> MVVKASGGSSVARPQLYQTVPVSTIIQAEQQDRFLNRGELDELAVYLRSGAKRLEIATTLTRNADIIVSRAANRIFVGGSPMAFLSRPQTEEAPQFTTGARGEAIDIKEAMKLGTATYVDTRGGFLEGLRSIFSASSGGAPVGFKPINIARYGPARMEKSLRDLDWFLRYTTYAIVAGDPNILAVNTRGLREIIEAACSSDATIAALQEMRRAALSYFEKDAEAKGIVETYFDVLINEFIAPAPSDKVRQRNSTDLQGLQLPQIYFNAAERRPKFVMKPGLSA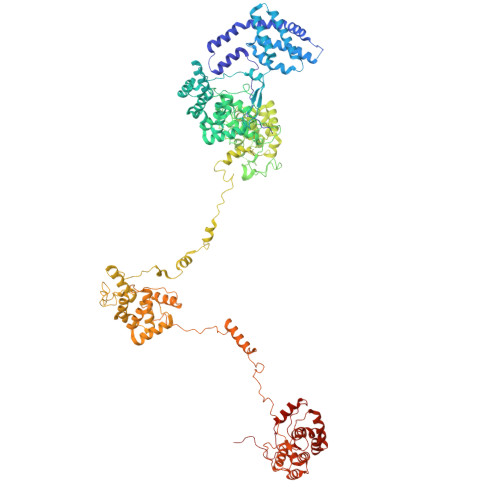AEKNEVVKAAYRQIFERDISRAYGLGISDLESKVKNGSISMKEFIRQLAKSPLYRKNFYEPYINSRALELAFRHILGRGPSSREEVQTYFAIISKGGLPALVDALVDSKEYSDYFGEETVPYLRGLGQEAQECRNWGAQQDLFKYSAPFRKVPQFITTFAAQDQPLPDQHPYGSGNDPLEIQFGAIFPKEKKNPSARPQPFNKDTRRILIARGPGINNQVSNPGARGLTPGTLGPKVFKLDQLPSINARIGKRSIATGTDSVKFAESSTQRVIRAAYLQVFGRDVYEGQRQKVAEIKLENGEISVREFVRILAKSNLFRSLYWTPLYVTKAIEYIHRRLLGRPTYGRQEMNAYFDIASKKGLYGLVDAIIDSQEYSEAFGEDTVPYERYITPQGLALRSLRVGTIGETGVPPEKEETPRFVELGAVTELRTEPAIQFRANQGVSKRREQTKVFKLTDLNDKQNLQLVIQAAYRQVFERDVAPYIVRDEFTALESKLSNGEITLKEFIEALGCSELYQKEFYTPYPNTKVIELGTKHFLGRAPLDQAEIRRYNQILATQGLKAFVQALVSSAEYAQAFGEDTVPYRRFPTLPAANFPNTEKLHNQLTKQSDAIVVPSFAPVKPRLDNTKLPLLSRAIAEQEAKARQADPSKPRFIELGRSFRNGDGQSVEVGVGTTRRRPARIFRMTVGAPSAEVELVINAIYCQVMDVFSGQVPSQFRRPDLESRLRNGEITVREFVRTLASSEIYRNRFYTPYPNTKVIEFLFRHLLGRAPATQAEIRQYNKILADQGLKTAVETMVNSPEYSRYFGEDVVPYKRFPTLPAGNYIGSVKADADLVKQSWSSLSPSLVGIQPSHRD> MHHHHHHGGGSENLYFQSDDKELIEYFKSQMKEDPDMASAVAAIRTLLEFLKRDKGETIQGLRANLTSAIETLCGVDSSVAVSSGGELFLRFISLASLEYSDYSKCKKIMIERGELFLRRISLSRNKIADLCHTFIKDGATILTHA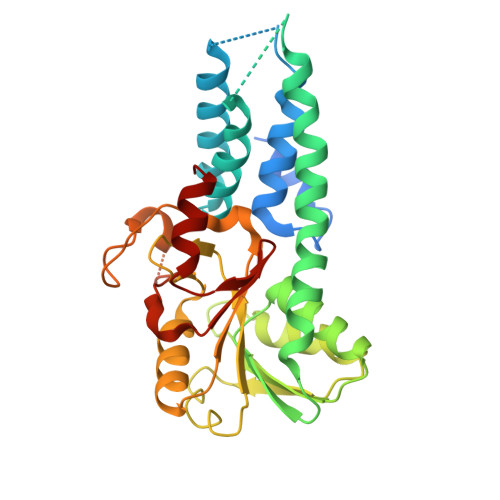YSRVVLRVLEAAVAAKKRFSVYVTESQPDLSGKKMAKALCHLNVPVTVVLDAAVGYIMEKADLVIVGAEGVVENGGIINKIGTNQMAVCAKAQNKPFYVVAESFKFVRLFPLNQQDVPDKFKYKADTLKVAQTGQDLKEEHPWVDYTAPSLITLLFTDLGVLTPSAVSDELIKLYL8-[(3~{R})-3-azanylpiperidin-1-yl]-7-[(2-bromophenyl)methyl]-1,3-dimethyl-purine-2,6-dione 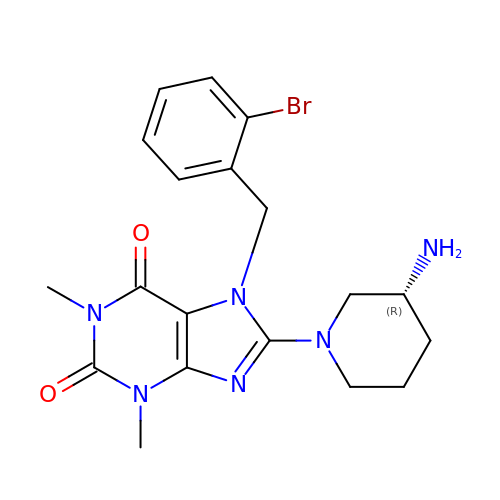| C19 H23 Br N6 O2 | CADOMWLQFMIXFQ-CYBMUJFWSA-N8-fluoranyl-5-methyl-1,2,3,6-tetrahydro-1,5-benzodiazocin-4-one 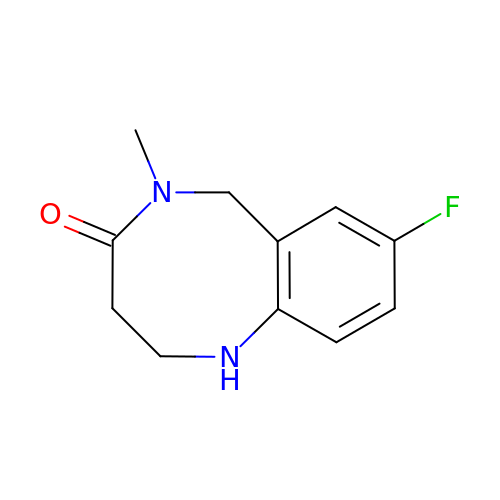| C11 H13 F N2 O | REEMTHAONJXYIX-UHFFFAOYSA-N> LQVDIVPSQGEISVGESKFFLCQVAGMLPTCEISWFSPNGEKLTPNQQRISVVWNDDSSTLTIYNANIDDAGIYKCVVHGPQCP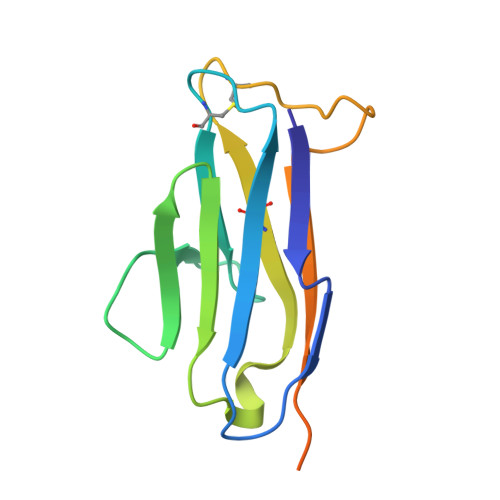RLTWSLGLPEATVNVKIFQGGGGSEQKLISEEDLSGENLYFQ> MSKSDYDSFYLSHFKYFLGPNPYLNTGALVFDFSISAPSKVLPLEDYHQEISQRFPQLESYPLTSYGELFAQTVAEVNQLEMDLHLNLYSIKDERIAVQSLDYQTSIEVVDLVWDWWEAITKDQRFNYQFRLKKAQETFRFSPYGGPSSYALIESAYKRKIPTFYLPEERLTQYGYGKYQIRGVSTTFNSDSHVDLDFTTVKDDCKGFLANCGFPVPQGYVVYSLREALNSAEDLGYPVVVKPVIGHKGIGVTANIENDKELEFA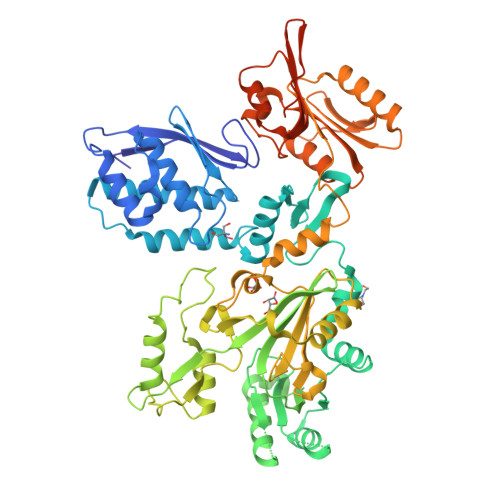YDRAVDASPNQRGQIIVEKYIPGADFRLLCVGGKFVAALERRPSYVIGDGRSTIYDLIEDENESPARQDTPTSALSPILIDKSLENYLEQQGLSLDSILERDRLVYLRKVANISAGGVSINVTPTIHPDNIILAEEIAQYFHIVCFGIDVISTDLSRSWKEGDFGIIEINAAPGIFMHLKPAIGDSIDVPGKILDYLFVSESTSRMPIITFNYLPKQTLLEIVNLVLQSHPHWTVGSICQDGMWINKSPKPLPKDYNTGVLTLLRHPKLDLLIAEYSQDIFETEGMLYEGSDLIILDEPTETEKILARDLRKEGILITKQENQVLIQRAEEQENYQLDELTSLSNLYEKQIYHLFERAENLYFQ> SMDPPPSETHKLVVVGGGGVGKSALTIQFIQSYFVSDYDPTIEDSYTKICSVDGIPARLDILDTAGQEEFGAMREQYMRAGHGFLLVFAINDRQSFNEVGKLFTQILRVKDRDDFPVVLVGNKADLESQRQVPRSEASAFGASHHVAYFEASAKLRLNVDEAFEQLVRA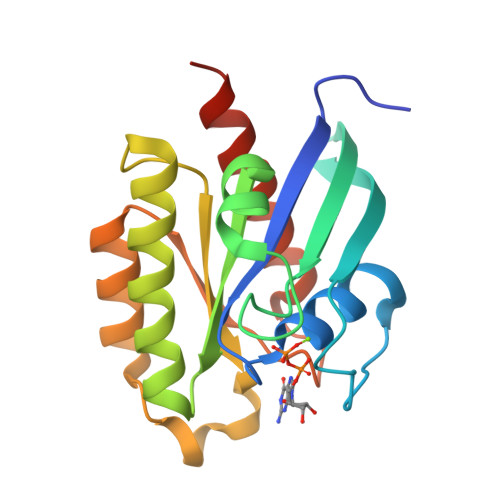VRKYQEQELPPS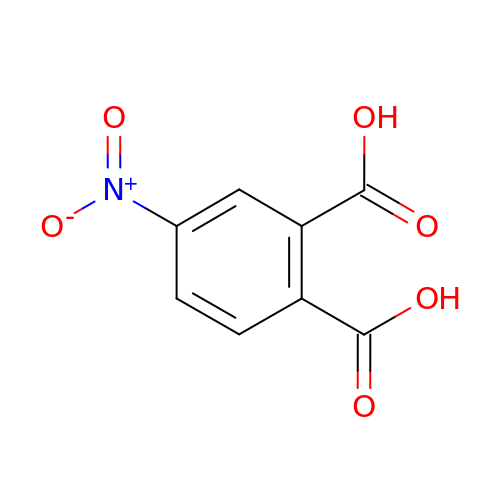4-nitrobenzene-1,2-dicarboxylic acid | C8 H5 N O6 | SLBQXWXKPNIVSQ-UHFFFAOYSA-N BBRF2 is an EBV tegument protein that has putative homologues in all three herpesvirus subfamilies. Here, we report crystal structures of BBRF2 alone and in complex with BSRF1. BBRF2 binds EBV capsid protein MCP and capsid-associated protein BPLF1, whereas BSRF1 associates with EBV glycoproteins gB and gH/gL. These data elucidate the molecular basis of the functional association between BBRF2 and BSRF1, suggesting a role of BBRF2-BSRF1 in tethering EBV nucleocapsids to the Golgi membrane during secondary envelopment.

Finally, we obtained crystals of the BBRF2Δ-BSRF1Δ complex and solved its structure at 3.1 Å. In the asymmetric unit, BBRF2Δ and BSRF1Δ formed a 6:6 heterododecamer. Using the PISA server, we found a predominantly large interface area of ~1300 Å2 between BBRF2Δ-1 and BSRF1Δ-1, which we think mediates the constitutive heterodimer observed in solution. Three constitutive heterodimers are associated in a symmetric manner to build up a triangular 3:3 heterohexamer. Two copies of the triangular 3:3 BBRF2Δ-BSRF1Δ heterohexamer stack face-to-face, resulting in a two-layer 6:6 heterododecamer in the asymmetric unit. The antiparallel ɑ6 and ɑ7 of BBRF2Δ join at the middle of ɑA and ɑB of BSRF1Δ, forming a tight heterogeneous four-helix bundle. A massive hydrophobic network stabilizes this helical bundle and constitutes the major interface of the BBRF2Δ-BSRF1Δ complex. Two bulky residues on ɑ7 of BBRF2Δ, Met205 and Phe209, wedge into the hydrophobic niche of BSRF1Δ, and hydrophobic residues from ɑ6 of BBRF2Δ add to this cluster. The proximal end of BSRF1Δ creates a hydrophilic interface with BBRF2Δ via two intermolecular salt bridges and a hydrogen bond. In addition, the N-terminal loop (N-loop) of BSRF1Δ winds toward the central β-sheet of BBRF2Δ, and a bulged 47-LPPGV-51 motif from the N-loop lies inside a hydrophobic groove.

>GPHMGGSMQKVSLRVTPRLVLEVNRHNAICVATNVPEFYNARGDLNIRDLRAHVKARMISSQFCGYVLVSLLDSEDQVDHLNIFPHVFSERMILYKPNNVNLMEMCALLSMIENAKSPSIGLCREVLGRLTLLHSKCNNLDSLFLYNGARTLLSTLVKYHDLEEGAATPGPWNEGLSLFKLHKELKRAPSEARDLMQSLFLTSGKMGCLARSPKDYCADLNKEEDANSGFTFNLFYQDSLLTKHFQCQTVLQTLRRKCLGSDTVSKIIP[6x];>[6x]GPLGSECPDRWRAEIDLGLPPGVQVGDLLRNEQTMGSLRQVYLLAVQANSITDHLKRFDAVRVPESCRGVVEAQVAKLEAVRSVIWNTMISLAVSGIEMDENGLKALLDKQAGDSLALMEMEKVATALKMD(2R)-3-[(R)-[(1S)-1-aminoethyl](hydroxy)phosphoryl]-2-methylpropanoic acid | C6 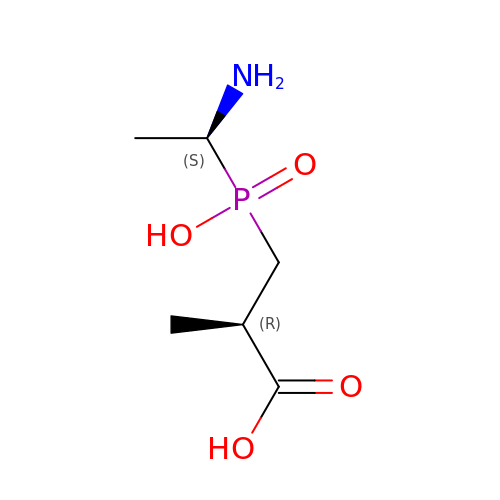H14 N O4 P | XXVGIEKADYFHOF-WHFBIAKZSA-N>[2x]SNAMKETVTML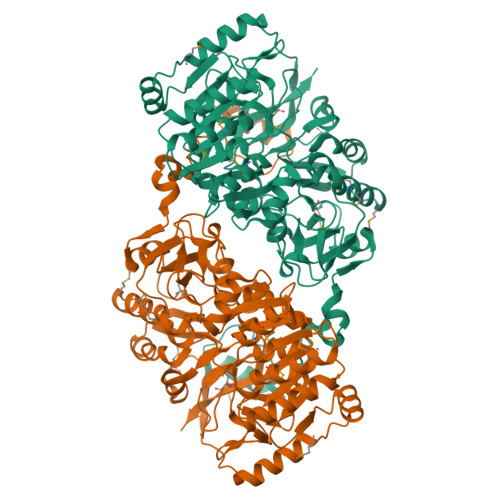NQQYVVPEGLQPYQGVTANSPWLASETEKRRRKICDSLEEAIRRSGLKNGMTISFHHAFRGGDKVVNMVMAKLAEMGFRDLTLASSSLIDAHWPLIEHIKNGVVRQIYTSGLRGKLGEEISAGLMENPVQIHSHGGRVKLIQSGELNIDVAFLGVPCCDEFGNANGFSGKSRCGSLGYAQVDAQYAKCVVLLTEEWVEFPNYPASIAQDQVDLIVQVDEVGDPEKITAGAIRLSSNPRELLIARQAANVIEHSGYFCDGFSLQTGTGGASLAVTRFLEDKMRRHNITASFGLGGITGTMVDLHEKGLIKALLDTQSFDGDAARSLAQNPHHIEISTNQYANPASKGAACERLNVVMLSALEIDVNFNVNVMTGSNGVLRGASGGHSDTAAGADLTIITAPLVRGRIPCVVEKVLTTVTPGASVDVLVTDHGIAVNPARQDLLDNLRAAGVALMTIEQLQQRAEQLTGKPQPIEFTDRVVAVVRYRDGSVIDVIRQVKG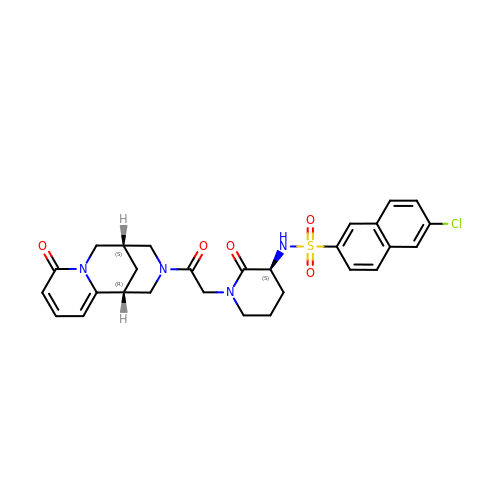6-chloro-N-((3S)-2-oxo-1-(2-oxo-2-((5S)-8-oxo-5,6-dihydro-1H-1,5-methanopyrido[1,2-a][1,5]diazocin-3(2H,4H,8H)-yl)ethyl)piperidin-3-yl)naphthalene-2-sulfonamide | C28 H29 Cl N4 O5 S | FLGSVBQCPOVGER-VNZMSGEBSA-N>MESKALLLLALSVCLQSLTVSRGGLVAADRITGGKDFRDIESKFALRTPEDTAEDTCHLIPGVTESVANCHFNHSSKTFVVIHGWTVTGMYESWVPKLVAALYKREPDSNVIVVDWLSRAQQHYPVSAGYTKLVGQDVAKFMNWMADEFNYPLGNVHLLGYSLGAHAAGIAGSLTNKKVNRITGLDPAGPNFEYAEAPSRLSPDDADFVDVLHTFTRGSPGRSIGIQKPVGHVDIYPNGGTFQPGCNIGEALRVIAERGLGDVDQLVKCSHERSVHLFIDSLLNEENPSKAYRCNSKEAFEKGLCLSCRKNRCNNMGYEINKVRAKRSSKMYLKTRSQMPYKVFHYQVKIHFSGTESNTYTNQAFEISLYGTVAESENI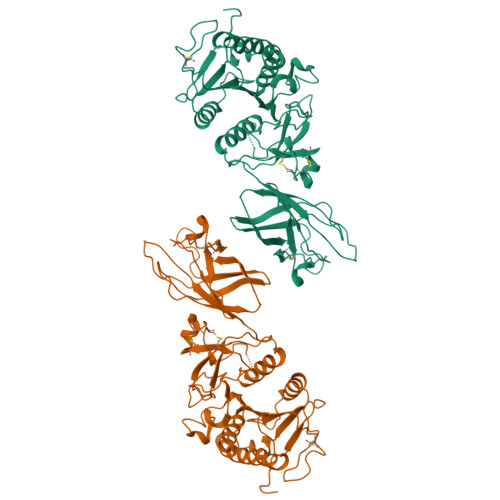PFTLPEVSTNKTYSFLLYTEVDIGELLMLKLKWISDSYFSWSNWWSSPGFDIGKIRVKAGETQKKVIFCSREKMSYLQKGKSPVIFVKCHDKSLNRKSG[2x]> DPSTYADYFSAWDKWEKQALPGEERDEAVSRLKECLINNSDELRLDRLNLSSLPDNLPAQITLLNVSYNQLTNLPELPVTLKKLYSASNKLSELPVLPPALESLQVQHNELENLPALPDSLLTMNISYNEIVSLPSLPQALKNLRATRNFLTELPAFSEGNNPVVREYFFDRNQISHIPESILNLRNECSIHISDNPLSSHALQALQRLTSSPDYHGPRIYFSMSD;> MDPMASEIHMTGPMCLIENTNGRLMANPEALKILSAITQPMVVVAIVGLYRTGKSYLMNKLAGKKKGFSLGSTVQSHTKGIWMWCVPHPKKPGHILVLLDTEGLGDVEKGDNQNDSWIFALAVLLSSTFVYNSIGTINQQAMDQLYYVTELTHRIRSKSSPDENENEVEDSADFVSFFPDFVWTLRDFSLDLEADGQPLTPDEYLTYSLKLKKGTSQKDETFNLPRLCIRKFFPKKKCFVFDRPVHRRKLAQLEKLQDEELDPEFVQQVADFCSYIFSNSKTKTLSGGIQVNGPRLESLVLTYVNAISSGDLPCMENAVLALAQIENSAAVQKAIAHYEQQMGQKVQLPTETLQELLDLHRDSEREAIEVFIRSSFKDVDHLFQKELAAQLEKKRDDFCKQNQEASSDRCSALLQVIFSPLEEEVKAGIYSKPGGYRLFVQKLQDLKKKYYEEPRKGIQAEEILQTYLKSKESMTDAILQTDQTLTEKEKEIEVERVKAESAQASAKMLHEMQRKNEQMMEQKERSYQEHLKQLTEKMENDRVQLLKEQERTLALKLQEQEQLLKEGFQKESRIMKNEIQDLQTKMRRRKACTIS

IpaH9.8 is one of the most well-studied members of the IpaH family and is secreted by Shigella flexneri during infection. IpaH proteins function as E3 ligases and subvert the host UPS pathway to suppress the host inflammasome and innate immune responses. Recently, it has been reported that IpaH9.8 targets human guanylate-binding protein 1 (hGBP1) for ubiquitination and degradation in order to suppress host defense in cells. In this study, we illuminated the key role of the LRR domain in autoinhibition of IpaH9.8 and revealed that IpaH9.8 can be activated by its LRR domain through substrate binding.

Crystals were obtained for the complex of the IpaH9.8 LRR domain and the full-length hGBP1, and the structure of the IpaH9.8LRR–hGBP1 complex was determined at 3.72 Å. The complex crystals belong to a space group P6122 and contained one heterodimer in each asymmetric unit. Structural analysis of the hGBP1/IpaH9.8LRR interface in both complex structures of IpaH9.8LRR–hGBP1 and IpaH9.8LRR–hGBP1LG-MD revealed that hGBP1 mainly interacted with the LRR-NT of IpaH9.8, rather than LRR-CT. Similar to the IpaH9.8LRR–hGBP1LG-MD complex, the LG domain of hGBP1 in the IpaH9.8LRR–hGBP1 complex interacted with the concave side of the IpaH9.8LRR mainly through the P-loop, the Switch II, and the α3 helix. However, the IpaH9.8LRR–hGBP1LG-MD structure lacks a GDP molecule that was observed at the catalytic center of the LG domain in the IpaH9.8LRR–hGBP1 complex. In the IpaH9.8LRR–hGBP1 complex, the guanine-cap was visible and revealed a similar orientation to other nucleotide-bound structures of hGBP1, and the phosphate-cap was also visible but flipped compared with other nucleotide-bound hGBP1 structures. This difference may have been caused by the lack of phosphate, which would normally bind to the phosphate cap. In addition, the α12 of the hGBP1-GED domain in IpaH9.8LRR–hGBP1 rotated ~10° with respect to hGBP1-apo (right). Indeed, in the IpaH9.8LRR–hGBP1 complex, the Glu147 of hGBP1 formed hydrogen-bond interactions with the Arg166 of IpaH9.8LRR (top), triggering main chain conformational changes in Arg166 and two other adjacent residues. Altogether, these results demonstrated that substrate-binding induced conformational changes in LRR-CT, which resulted in destabilization of the hydrophobic cluster and LRR-CT, which could disrupt the LRR–NEL interaction.> MVIVPEGTQLDEKQHIVINNGAEPQSFDPHKTEGVPESNVAYQLLEGLVTSDSEGKLQPGAAESWENTPDFKTWTFHLRKDAKWSNGDPVTAHDFVFAW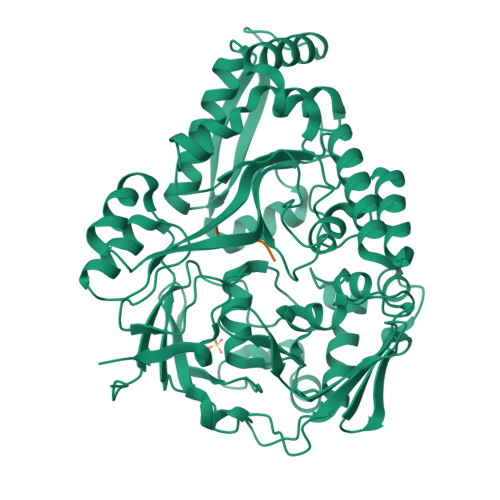RRLVDPATAAPYASYLSYLQVENAQDIIDGKKKPAELGVEAKDDYTFVVHATNPVPYAVSLTTHQSLLPLPQKVVEKLGDAWVKKENYVGNGAYKLANHIINEKIEFERNPLYWNDKETVINSATFLAIENPSTDVARYRAGDLDMTSYGLPPEQFAKLKKELLGEVYVTRTLGTYSYELNNKKAPFDNVNIRKALNLSLDRNVITDKVLGQGQTPTYVFTPTYIEEGHLIQQPAYSKEPMAQRNEEAIKLLEEAGYSKANPLKFSILYNTNENHKKVAIAAASMWKANTKGLIDVKLENQEWKTYIDSRRAGRYDVARAGWHADYNQATTFGNYFLSNSSNNTAKYANPEYDKAMAESYAATDAEGRAKAYAKAEEILGKDYGIVPIFNYVNPRLVKPYVKGYSGKDPQDHIYLRNLYIIKHLEHHHHHH;> RPPGF> FPELKNDTFLRAAWGEETDYTPVWCMRQAGRYLPEFRETRAAQDFFSTCRSPEACCELTLQPLRRFPLDAAIIFSDILVVPQALGMEVTMVPGKGPSFPEPLREEQDLERLRDPEVVA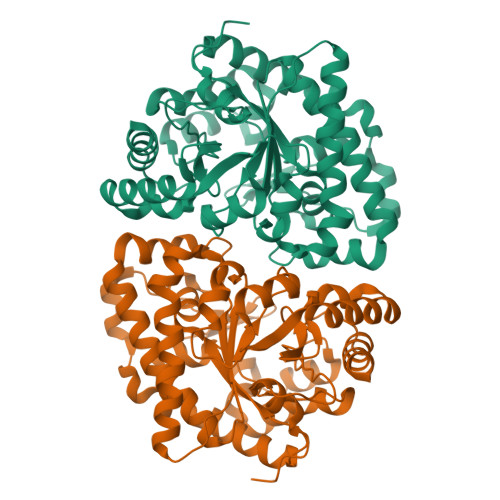SELGYVFQAITLTRQRLAGRVPLIGFAGAPWTLMTYMVERGGSSTMAQAKRWLYQRPQASHQLLRILTDALVPYLVGQVVAGAQALQLFESHAGHLGPQLFNKFALPYIRDVAKQVKARLREAGLAPVPMIIFAKDGHFALEELAQAGYEVVGLDWTVAPKKARECVGKTVTLQGNLDPCALYASEEEIGQLVKQMLDDFGPHRYIANLGHGLYPDMDPEHVGAFVDAVHKHSRLLRQ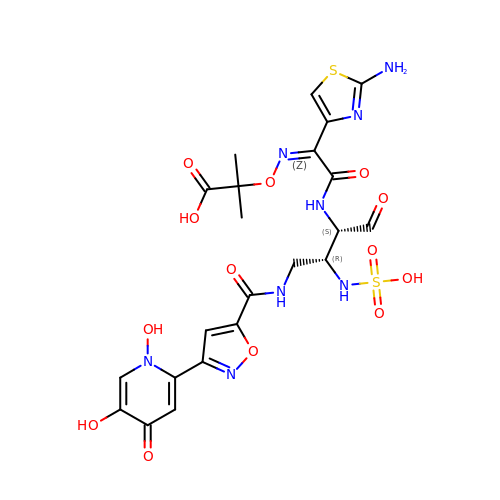(4R,5S,8Z)-8-(2-amino-1,3-thiazol-4-yl)-1-[3-(1,5-dihydroxy-4-oxo-1,4-dihydropyridin-2-yl)-1,2-oxazol-5-yl]-5-formyl-11,11-dimethyl-1,7-dioxo-4-(sulfoamino)-10-oxa-2,6,9-triazadodec-8-en-12-oic acid | C22 H24 N8 O13 S2 | OFOVQVNKWTUULV-NEEHKMPWSA-N> MNVLNRRQALQRALL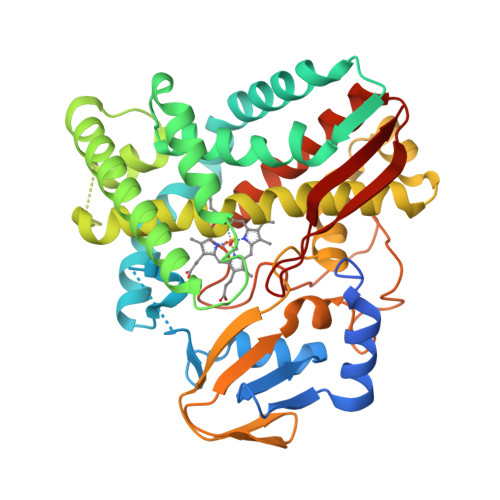NGKNKQDAYHPFPWYESMRKDAPVSFDEENQVWSVFLYDDVKKVVGDKELFSSCMPQQTSSIGNSIINMDPPKHTKIRSVVNKAFTPRVMKQWEPRIQEITDELIQKFQGRSEFDLVHDFSYPLPVIVISELLGVPSAHMEQFKAWSDLLVSTPKDKSEEAEKAFLEERDKCEEELAAFFAGIIEEKRNKPEQDIISILVEAEETGEKLSGEELIPFCTLLLVAGNETTTNLISNAMYSILETPGVYEELRSHPELMPQAVEEALRFRAPAPVLRRIAKRDTEIGGHLIKEGDMVLAFVASANRDEAKFDRPHMFDIRRHPNPHIAFGHGIHFCLGAPLARLEANIALTSLISAFPHMECVSITPIENSVIYGLKSFRVKM> LGNVVCVTGASGYIASWLVRLLLHRGYTVKATVRDPNDPKKVDHLVKLDGAKERLQLFKANLLEEGAFDSVVQGCHGVFHTASPFYHDVKDPQAELIDPALKGTLNVLNSCAKSPSLKRVVLTSSIAAVAYNGKPRTPDVVVDETWFTDADFCAKSNLWYVVSKTLAEEAAWKFVKENNIDMVTINPAMVIGPLLQPVLNTSAAAILNLINGAQTFPNASFGWVNVKDVANAHILAYENASASGRHCLVERVAHYSEVVRILRELYPSLQLPEKCA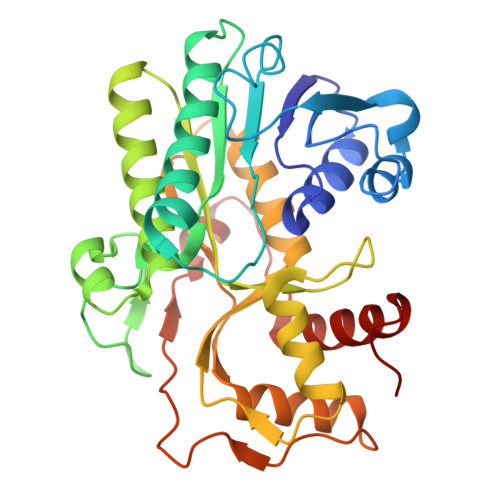DDKPYVPIYQVSKEKAKSLGLEYTPLEVSIKETVESLKEKKFANL>MSEGQIPSSDVLGSQLGVGVQGASLYCPQENYTTKKQEKPQWLRPVDDTLAEDALDLHIVVKSLLCDTAIRYISDDKVLQESDADDDLITSDIDEDTDNQGDTSIVVNPVIPVVPKDVHFFKKVDVGNDSMFGVNCDTPVSFQDYIPSDLLRNLDDTLQESTNSSRPMQDAFFWDPTVANRLDSQYIQTASDLRNYRDGTEIIAYASGKTGSVLNIAVLTRQNTLHLNRHNNVTSIELHSPIKSIKIPGASESIGRRSNLVGIITENSFQIFRIESVHSRSCDVMVSSSEPLYFVEIDDLQVVDFAFNPWDLQQFAIIDIKGNWSIGRIPKNFNNNNKRKLQLIDNLHGTIFDPEELSSWKRIEWFSHFQKILVFDRSKMIEIDFMNNWQTEVVQAKAWSNIRDYKRIDDKNGILLTSREIIIVGASESNDPVRRISWKHDLDPDDTTLRITVQKVKKPDHILLVAFVYSMRHKRIYMHVFSHRKANLFQSLGCSTVLEIPGGTPTGIETILTLDHIDDESRREEDADENFELVVDFLVKLRNSSEVYYYALSNTQNSEPNKQETPIIVDHPEWASLFNNADEREKESIGALVSQIKLKERERISRVQNLIEHENSHDEDKYLQDLGYRLSIATNELLESWQKTKDESILSGSLSHSKLKNLLENSDSFASIPEFSSLLDQFFQYYQDQDVTFIGFEKLLHLFLHEDVPGLDIFYNKLLQCWVLVSPQAELLTKEIVKDIIWSLARLEKPSLFEPIQNEISRSLSGPYQDIISSWDMDDINEEDESNEFNFDSQFSAPFNGRPPFNLNSQSQIPTIKSSQSSGLARRKRILKTQSQKATPLSQSTQNLSVLPDSMTPAFTLMQPPSSQISFVNDSQPRNSQKAKKKKKRIRGFG[6x];>MSTFIRGPICGTDNCPSRLWRIIDGRRTCQYGHVMEGDVEFNDDEDDLNGLGAGVITRRLNLTTNATGSFQSSQLTNSQLLQQQQRQSHKKFKKLIGHEAKLLFLKSFQFILKRQIRWLITEMRFPKEFEHVAKIIWLKILKTINDQPQEELKLQLHMTSTISILYLASTHLSLPVYTCDYIKWICTAKMPYFQASEILPKSWRIQLPNYYVSILEGSISPFNGQLYNKIALTCGMIHFKEFFNSEISCQGLLLKLVMQCALPPEFYFYTKQVIEFEETDIRNLTLWERTDERHTGRVSNHAELRVLSYFMLTINWMLSFDRDRQYPLKWILSLTESLTQRTTTSESIGRNIVKVVYPDKPTSSDYFQWSEEETLEFLKWMEKQFLPTQTKSLHNENGSMEMTIDQKIARRKLYKIFPLDREANHDGEFNDSTHQLTFIEDLQERYAKQTPFFESNKIRDSLNYQEANPPARKEAIGRLLTHIASQLLVDFAISKEQLKDCISRIKNACLHRMN[6x];>MFEVPITLTNRKFAQRRKLKYQYINYISRRFDRISKKSTTTDSLPTPENSAAENNDEEEGQNSEAGTYRRSVLQQKKRRRERHWRSVVGEIYSTTESETDSQEEETEEGGEHDTGIDKEDSDEERKFWKKYEKPEKSFEIWRTVSSQNKQPINKQKMTYHNFKKIEKIPLRKMEIPLLHCTKENKLYFQSISRGLEPLKTSTSEVRNYRTRHIVTLTDLLHLNVSRHNWSLAYKIFATLIRIPGVQIKSLWGIGVEILDNLSNSSSGLDFLQWMCQIYSSKSRFVQNINYRSIVPPFQTGSRTHTAKFAITYLWSSLINCQKSMEPSSNIIDKPFDTENDLLQELIDKISEWVLTPP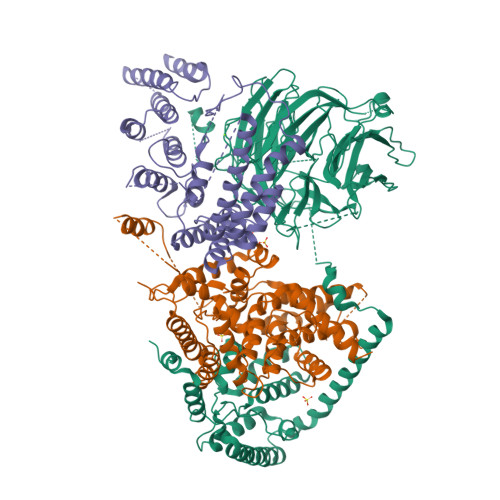FMEDAEVWFIYASCHLLKADTLSRQFVNDNKNNDLIGLDRDIKINQVIKHIHYVRTFLKICLDKGGFAVPSRLIENQLKSFESRLYGEAQDIQERDVANVYDSIDNSSVENSFGDVYETNAEFLDTQLMDLSPEDNGLDEMHYSDEDSSE[6x]cyclopropyl-[1-(2-fluoranylethyl)-5-[[4-[4-[[(3~{R},4~{S})-3-methoxy-4-oxidanyl-pyrrolidin-1-yl]methyl]-3-methyl-pyrazol-1-yl]pyrimidin-2-yl]amino]indol-3-yl]methanone 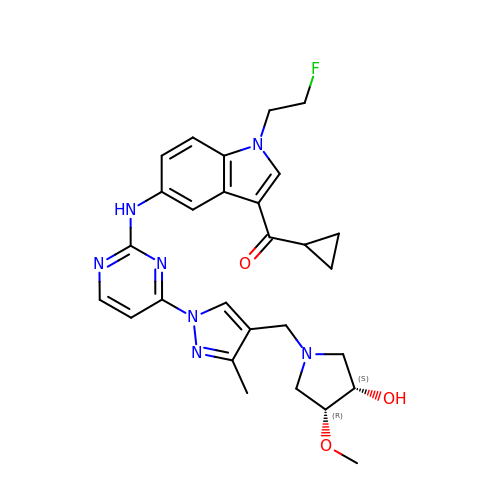| C28 H32 F N7 O3 | BOEORZOOBBGDDF-LOSJGSFVSA-N>EEDKAYWNKDAQDALDKQLGIKLREKQAKNVIFFLGDGMSLSTVTAARIYKGGLTGKFEREKISWEEFDFAALSKTYNTDKQVTDSAASATAYLTGVKTNQGVIGLDANTVRTNCSYQLDESLFTYSIAHWFQEAGRSTGVVTSTRVTHATPAGTYAHVADRDWENDSDVVHDREDPEICDDIAEQLVFREPGKNFKVIMGGGRRGFFPEEALDIEDGIPGEREDGKHLITDWLDDKASQGATASYVWNRDDLLAVDIRNTDYLMGLFSYTHLDTVLTRDAEMDPTLPE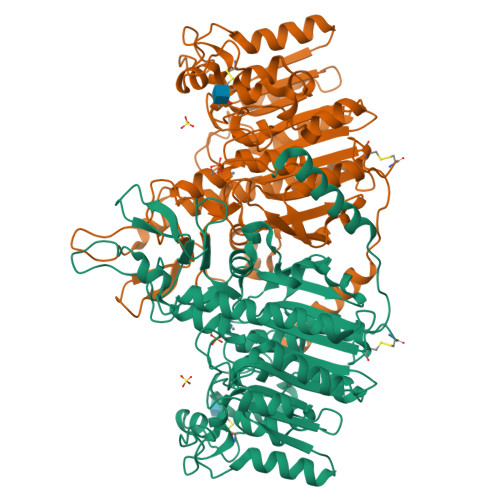MTKVAIEMLTKDENGFFLLVEGGRIDHMHHANQIRQSLAETLDMEEAVSMALSMTDPEETIILVTADHGHTLTITGYADRNTDILDFAGISDLDDRRYTILDYGSGPGYHITEDGKRYEPTEEDLKDINFRYASAAPKHSVTHDGTDVGIWVNGPFAHLFTGVYEENYIPHALAYAACVGTGRTFCDEK[2x]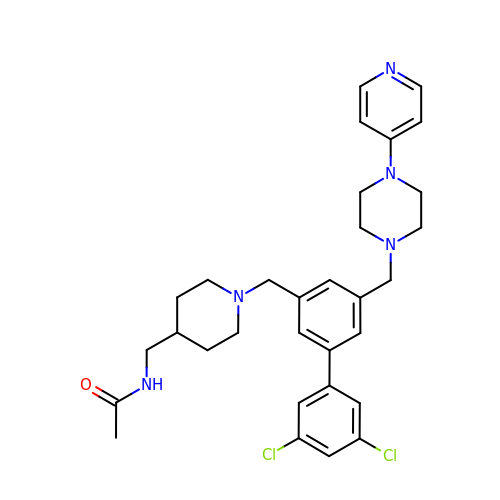~{N}-[[1-[[3-[3,5-bis(chloranyl)phenyl]-5-[(4-pyridin-4-ylpiperazin-1-yl)methyl]phenyl]methyl]piperidin-4-yl]methyl]ethanamide | C31 H37 Cl2 N5 O | SNVXMRYCRVZGRY-UHFFFAOYSA-N> PFKIFKASPPPAPTGRKPTGYRGNHWHKKVLYDPVYPTTKVPAALVPRYPIDWRNGGRALLIAALSKLEGASALQRRIFLRENSRESQVPQTPLSPFQTGSSASGGGAYLVSSLGRKRSYVGRIAVSLMPRHRQIADYQRVGGFCSPRCFSECSKELRRCLCAWRCTGFHEHVVQMDGM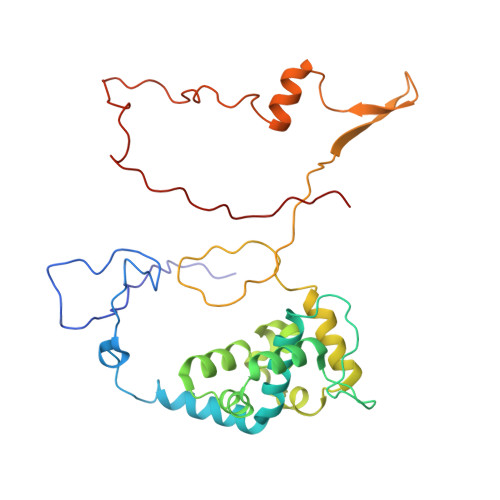LGEYKGEVKTEKPLFSVLRRQARRNADPSEGVAFCAESAKFKSVRRAQHPAFEAFDRQGPDGPSQKPAPRKEPPLPFYSASHVPNVPRPPPPQPYTGPLKVREG> KQYPIINFTTAGATVQSYTNFIRAVRGRLTTGADVRHEIPVLPNRVGLPINQRFILVELSNHAELSVTLALDVTNAYVVGYRAGNSAYFFHPDNQEDAEAITHLFTDVQNRYTFAFGGNYDRLEQLAGNLRENIELGNGPLEEAIS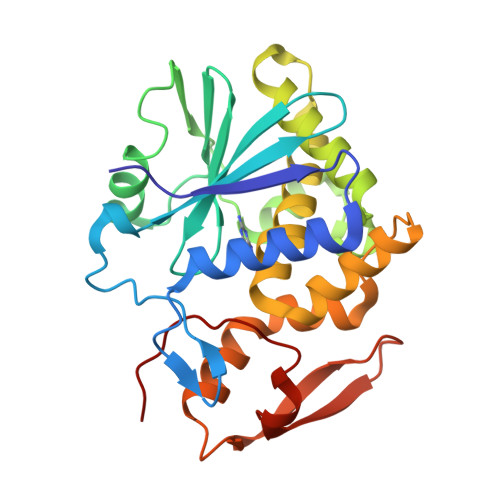ALYYYSTGGTQLPTLARSFIICIQMISEAARFQYIEGEMRTRIRYNRRSAPDPSVITLENSWGRLSTAIQESNQGAFASPIQLQRRNGSKFSVYDVSILIPIIALMVYRCAP>[8x]MRGSHHHHHHGSFIDRVKALLGERVKDVRLTHRLTDTPAIVSTDADEMSTQMAKLFAAAGQKVPEVKYIFELNPDHVLVKRAADTEDEAKFSEW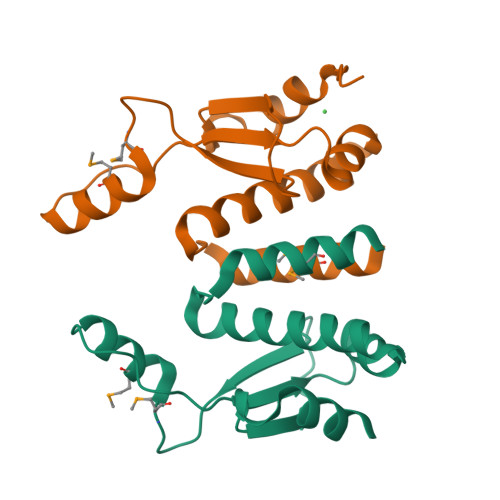VELLLDQALLAERGTLEDPNLFIRRMNQLLVS> MDCYRTSLSSSWIYPTVILCLFGFFSMMRPSEPFLIPYLSGPDKNLTSAEITNEIFPVWTYSYLVLLLPVFVLTDYVRYKPVIILQGISFIITWLLLLFGQGVKTMQVVEFFYGMVTAAEVAYYAYIYSVVSPEHYQRVSGYCRSVTLAAYTAGSVLAQLLVSLANMSYFYLNVISLASVSVAFLFSLFLPMPKKSMFFHAKPSREIKKSSSVNPVLEETHEGEAPGCEEQKPTSEILSTSGKLNKGQLNSLKPSNVTVDVFVQWFQDLKECYSSKRLFYWSLWWAFATAGFNQVLNYVQILWDYKAPSQDSSIYNGAVEAIATFGGAVAAFAVGYVKVNWDLLGELALVVFSVVNAGSLFLMHYTANIWACYAGYLIFKSSYMLLITIAVFQIAV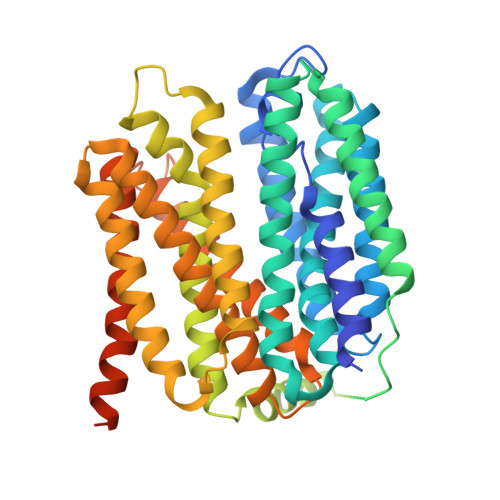NLNVERYALVFGINTFIALVIQTIMTVIVVDQRGLNLPVSIQFLVYGSYFAVIAGIFLMRSMYITYSTKSQKDVQSPAPSENPDVSHPEEESNIIMSTKL> KETAAAKFERQHMDSSTSAASSSNYCNQMMKSRNLTKDRCKPVNTFVHESLADVQAVCSQKNVACKNGQTNCYQSYSTMSITDCRETGSSKYANCAYKTTQANKHIIVACEGNPYVPVH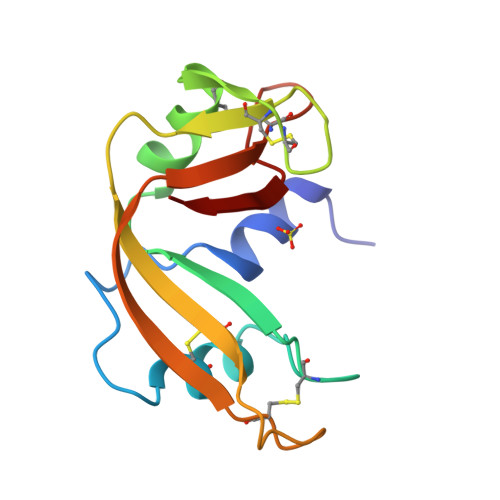FDASV1-[4-chloranyl-2,6-di(propan-2-yl)phenyl]-3-[4-(2-oxidanylpropan-2-yl)furan-2-yl]sulfonyl-urea | C20 H27 Cl N2 O5 S | 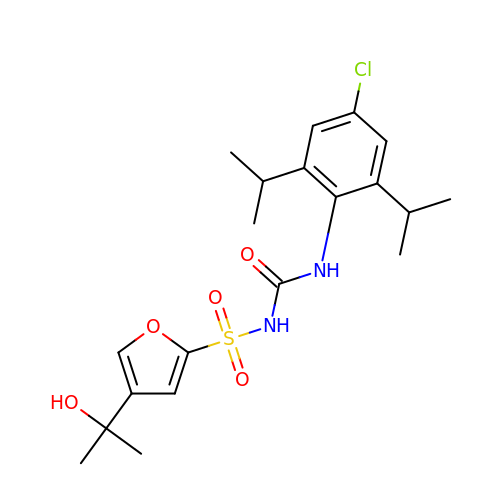RTJGVFANTDWUEG-UHFFFAOYSA-N> GANSLSVHQLAAQGEMLYLATRIEQENVINHTDEEGFTPLMWAAAHGQIAVVEFLLQNGADPQLLGKGRESALSLACSKGYTDIVKMLLDCGVDVNEYDWNGGTPLLYAVHGNHVKCVKMLLESGADPTIETDSGYNSMDLAVALGYRSVQQVI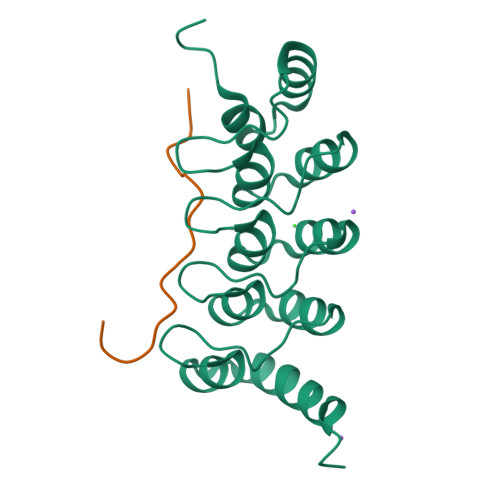ESHLLKLLQNIKE;> XLPLYTSPSLPNITLGLP> MFKAQATFSRYSAAVSLLLLFSGAAQAAPQSITTLPLQPDGENRWRLPAGEYQGQFTIEQPMQLRCEPGAVIQSQGQGSSLLISAPDVLVEGCTLYEWGSDLTAMDSAVFILPAAERAQISNNRMRGPGFGVFVDGTRDVQVIGNEIDGDAGVRSQDRGNGIHLFAVSGARVLHNHVRNARDGIYIDTSNGNHLEGNVIEDVRYGVHYMFANENSLIDNVTRRTRTGYALMQSRKLTVTGNRSEQDQNYGILMNYITYSTITGNFVS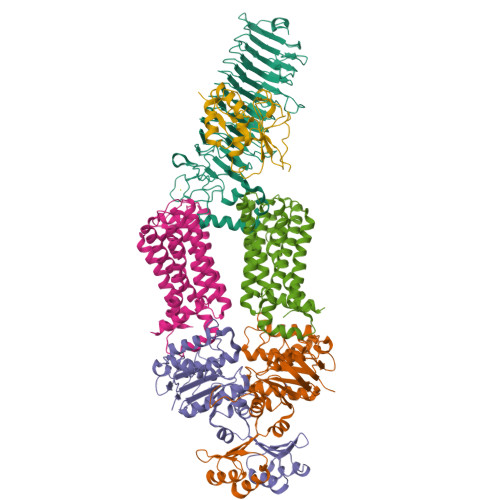DVQRGDTGGDSMISGGEGKALFIYNSLFNTIENNHFEKSSLGIHLTAGSEDNRISGNAFVGNQQQVKYVASRTQEWSVDGRGNYWSDYLGWDRNNDGLGDIAYEPNDNVDRLLWLYPQVRLLMNSPSIEVLRWVQRAFPVIKSPGVQDSHPLMKLPTEKLLTEKQEPTS;>[2x]MNAVEIQGVSQRYGSMTVLHDLNLNLGEGEVLGLFGHNGAGKTTSMKLILGLLSPSEGQVKVLGRAPNDPQVRRQLGYLPENVTFYPQLSGRETLRHFARLKGAALTQVDELLEQVGLAHAADRRVKTYSKGMRQRLGLAQALLGEPRLLLLDEPTVGLDPIATQDLYLLIDRLRQRGTSIILCSHVLPGVEAHINRAAILAKGCLQAVGSLSQLRAEAGLPVRIRASGISERDSWLQRWTDAGHSARGLSESSIEVVAVNGHKLVLLRQLLGEGEPEDIEIHQPSLEDLYRYYMERAGDVRAQEGRL;>MNQVWNIARKELSDGLRNRWLLAISLLFAVLAVGIAWLGAAASGQLGFTSIPATIASLASLATFLMPLIALLLAYDAIVGEDEGGTLMLLLTYPLGRGQILLGKFVGHGLILALAVLIGFGCAALAIALLVEGVELGMLFWAFGRFMISSTLLGWVFLAFAYVLSGKVNEKSSAAGLALGVWFLFVLVFDLVLLALLVLSEGKFNPELLPWLLLLNPTDIYRLINLSGFEGSGSAMGVLSLGADLPVPAAVLWLCLLAWIGVSLLLAYAIFRRRLT[2x];> MNALHRIGAGTLLAVLLAFGLTGCGEKEEVQQSLEPVAFHDSDECHVCGMIITDFPGPKGQAVEKRGVKKFCSTAEMLGWWLQPENRLLDAKLYVHDMGRSVWEKPDDGHLIDATSAYYVVGTSLKGAMGASLASFAEEQDAKALAGMHGGRVLRFEEIDQALLQEAASMQHGGMHDHAPNGAHNAHAGH NOD1 and NOD2 (Nucleotide-binding oligomerization domain-containing proteins 1 and 2) are cytosolic receptors of the innate immune system, which respond to intracellular fragments of the bacterial peptidoglycans, D-glutamyl-meso-diaminopimelic acid (iE-DAP) and muramyl dipeptide (MPD), respectively. Upon ligand recognition, NOD receptors oligomerise and recruit an adaptor protein, Receptor Interacting protein kinase 2 (RIP2), through interactions of their respective CARD domains. RIP2 also contains an N-terminal dual-specificity ser/tyr kinase domain (RIP2K), which belongs to the TKL kinase family (Tyrosine kinase-like). RIP2 undergoes auto-phosphorylation and K-63 linked ubiquitination at Lys209, becoming a scaffolding protein for downstream effectors.

We successfully crystallised and solved the structures of all three RIP2K samples: the structure of wild-type RIP2K with bound the ATP analogue AMPPCP (β,γ-methylene-adenosine 5′-triphosphate) (RIP2K-AMPPCP), the structure of RIP2KD146N within Staurosporine bound (RIP2KD146N -STAU) and the structure of RIP2KK47R. Crystals of RIP2KD146N have been obtained in the apo state and with AMP-PCP or the promiscuous inhibitor staurosporine bound, without significant differences in the resulting structures. The best crystals diffracted to 2.8 Å resolution and were obtained with staurosporine. Each monomer has an inhibitor molecule bound in the active site, whose configuration presents all the features of a kinase in the active state. Differently from the ligand in the RIP2K-AMPPCP structure, staurosporine is coordinated by Gln150 backbone, while Gln150 sidechain is hydrogen bonded to the Tyr192 phenyl ring in the AS. Differently from the IRAK4-KDD311N structure, we did not observe a possible prone-to-autophosphorylate conformation in cristallo. The AS is close to the loop containing the site of ubiquitination Lys209 (residues 200–210, referred to here as the Lys209 loop), which is also disordered. Both structures crystallised in the tetragonal space group P41212 with a dimer in the asymmetric unit, in agreement with the size exclusion chromatography profile. In agreement with the crystal structure, the data show that RIP2KD146N is a dimer. In support of this, AUC analyses show that RIP2KK47R has a tendency to form tetramers and RIP2KD146N structure show an active dimer without phosphorylation at AS.

>[2x]GAMAMNGEAICSALPTIPYHKLADLRYLSRGASGTVSSARHADWRVQVAVKHLHIHTPLLDSERKDVLREAEILHKARFSYILPILGICNEPEFLGIVTEYMPNGSLNELLHRKTEYPDVAWPLRFRILHEIALGVNYLHNMTPPLLHHNLKTQNILLDNEFHVKIADFGLSKWRMMSLSQSRSSKSAPEGGTIIYMPPENYEPGQKSRASIKHDIYSYAVITWEVLSRKQPFEDVTNPLQIMYSVSQGHRPVINEESLPYDIPHRARMISLIESGWAQNPDERPSFLKCLIELEPVLRTFEEI4-amino-5-chloro-2-{4-(1-beta-D-glucopyranuronosylpiperidin-4-yl)-5-methyl-2-[(propan-2-yl)oxy]anilino}pyrimidine 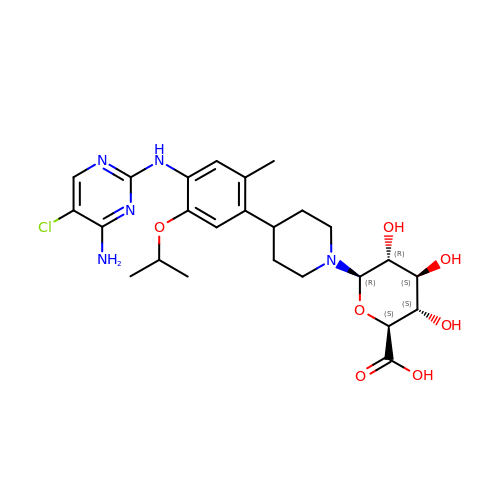| C25 H34 Cl N5 O7 | SFTKCGCNKCPXPY-KHYDEXNFSA-N> DDHSELLVNTKSGKVMGTRVPVLSSHISAFLGIPFAEPPVGNMRFRRPEPKKPWSGVWNASTYPNNCQQYVDEQFPGFSGSEMWNPNREMSEDCLYLNIWVPSPRPKSTTVMVWIYGGGFYSGSSTLDVYNGKYLAYTEEVVLVSLSYRVGAFGFLALHGSQEAPGNVGLLDQRMALQWVHDNIQFFGGDPKTVTIFGESAGGASVGMHILSPGSRDLFRRAILQSGSPNCPWASVSVAEGRRRAVELGRNLNCNLNSDEELIHCLREKKPQELIDVEWNVLPFDSIFRFSFVPVIDGEFFPTSLESMLNSGNFKKTQILLGVNKDEGSFFLLYGAPGFSKDSESKISREDFMSGVKLSVPHANDLGLDAVTLQYTDWMDDNNGIKNRDGLDDIVGDHNVICPLMHFVNKYTKFGNGTYLYFFNHRASNLVWPEWMGVIHGYEIEFVFGLPLVKELNYTAEEEALSRRIMHYWATFAKTGNPNEPHSQESKWPLFTTKEQKFIDLNTEPMKVHQ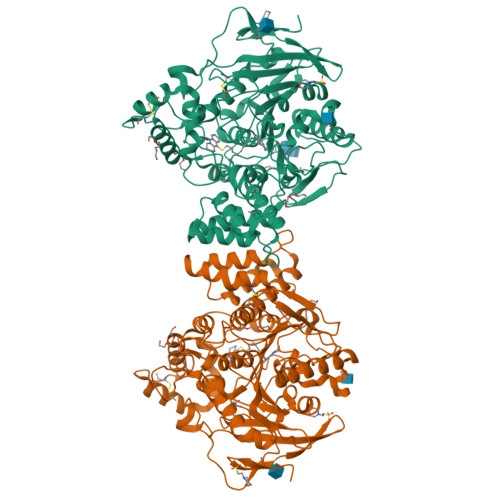RLRVQMCVFWNQFLPKLLNAT> MKTWLMGFSEFLLRYKLVWSETWKIRKQLDTPVREKDENEFLPAHLELIETPVSRRPRLVAYFIMGFLVIAVILSVLGQVEIVATANGKLTLSGRSKEIKPIENSIVKEIIVKEGESVRKGDVLLKLTALGAEADTLKTQSSLLQTRLEQTRYQILSRSIELNKLPELKLPDEPYFQNVSEEEVLRLTSLIKEQFSTWQNQKYQKELNLDKKRAERLTILARINRYENLSRVEKSRLDDFDDTLEVTALVQ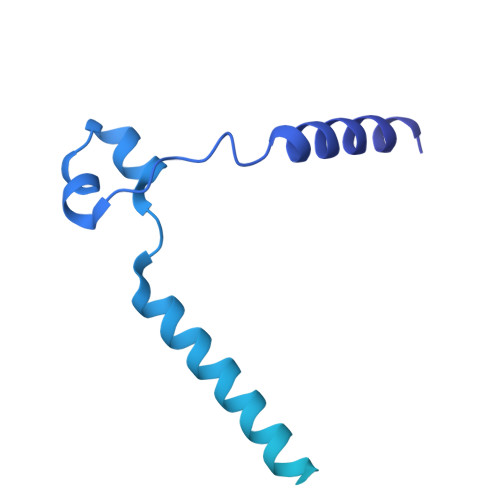NKDIGFINVGQNAIIKVEAFPYTRYGYLVGKVKNINLDAIEDQKLGLVFNVIVSVEENDLSTGNKHIPLSSGMAVTAEIKTGMRSVISYLLSPLEESVTESLHER> ANIVGGIEYSINNASLCSVGFSVTRGATKGFVTAGHCGTVNATARIGGAVVGTFAARVFPGNDRAWVSLTSAQTLLPRVANGSSFVTVRGSTEAAVGAAVCRSGRTTGYQ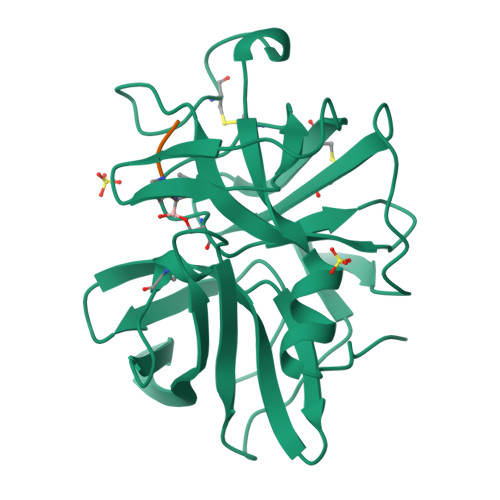CGTITAKNVTANYAEGAVRGLTQGNACAGRGDSGGSWITSAGQAQGVMSGLNVQSNGNNCGIPASQRSSLFERLQPILSQYGLSLVTG;> XAAPL> GPGVTEEQVH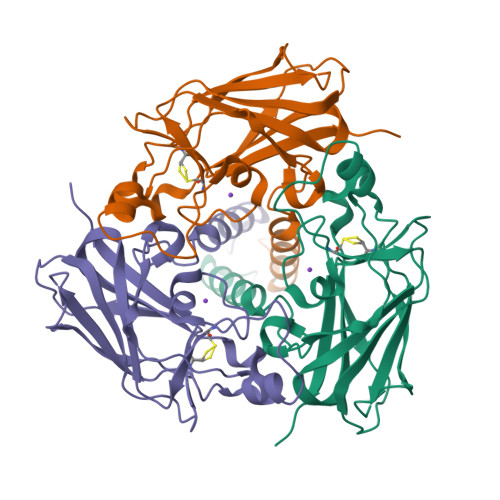HIVKQALQRYSEDRIGLADYALESGGASVISTRCSETYETKTALLSLFGIPLWYHSQSPRVILQPDVHPGNCWAFQGPQGFAVVRLSARIRPTAVTLEHVPKALSPNSTISSAPKDFAIFGFDEDLQQEGTLLGKFTYDQDGEPIQTFHFQAPTMATYQVVELRILTNWGHPEYTCIYRFRVHGEPAH> QDWLTFQKKHITNTRDVD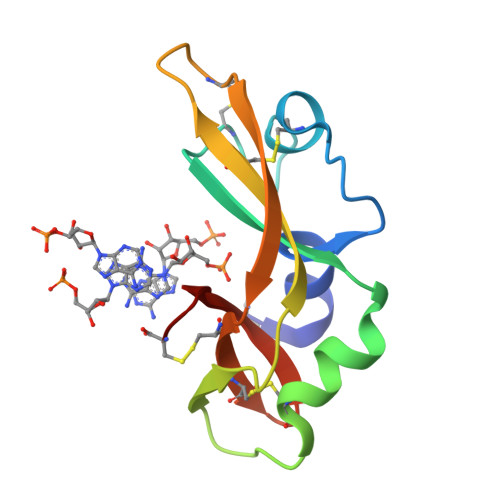CDNIMSTNLFHCKDKNTFIYSRPEPVKAICKGIIASKNVLTTSEFYLSDCNVTSRPCKYKLKKSTNKFCVNCANQAPVHFVGVGSC> EGPAKKVLTLEGDLVLGGLFPVHQKGGPAEDCGPVNEHRGIQRLEAMLFALDRINRDPHLLPGVRLGAHILDSCSKDTHALEQALDFVRASLSRGADGSRHICPDGSYATHGDAPTAITGVIGGSYSDVSIQVANLLRLFQIPQISY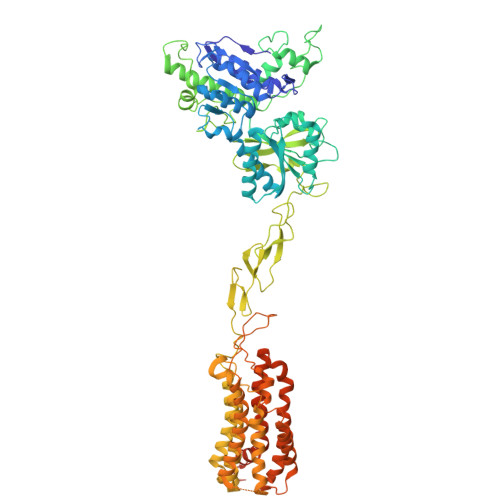ASTSAKLSDKSRYDYFARTVPPDFFQAKAMAEILRFFNWTYVSTVASEGDYGETGIEAFELEARARNICVATSEKVGRAMSRAAFEGVVRALLQKPSARVAVLFTRSEDARELLAASQRLNASFTWVASDGWGALESVVAGSEGAAEGAITIELASYPISDFASYFQSLDPWNNSRNPWFREFWEQRFRCSFRQRDCAAHSLRAVPFEQESKIMFVVNAVYAMAHALHNMHRALCPNTTRLCDAMRPVNGRRLYKDFVLNVKFDAPFRPADTHNEVRFDRFGDGIGRYNIFTYLRAGSGRYRYQKVGYWAEGLTLDTSLIPWASPSAGPLPASRCSEPCLQNEVKSVQPGEVCCWLCIPCQPYEYRLDEFTCADCGLGYWPNASLTGCFELPQEYIRWGDAWAVGPVTIACLGALATLFVLGVFVRHNATPVVKASGRELCYILLGGVFLCYCMTFIFIAKPSTAVCTLRRLGLGTAFSVCYSALLTKTNRIARIFGGAREGAQRPRFISPASQVAICLALISGQLLIVVAWLVVEAPGTGKETAPERREVVTLRCNHRDASMLGSLAYNVLLIALCTLYAFKTRKCPENFNEAKFIGFTMYTTCIIWLAFLPIFYVTSSDYRVQTTTMCVSVSLSGSVVLGCLFAPKLHIILFQPQKNVVSHRAPTSRFGSAAARASSSLGQGSGSQFVPTVCNGREVVDSTTSSL The HCV NS3/4A protease – a chymotrypsin-like serine protease – is a prime therapeutic target that cleaves four known sites along the virally encoded polyprotein. The NS3/4A protease also hydrolyzes two human proteins, TRIF and MAVS, which are part of the innate immune system, thereby confounding the innate immune response to viral infection. In this study, we report that four chemically representative protease inhibitors – telaprevir, danoprevir, vaniprevir and MK-5172 – exhibit distinct susceptibilities to the protease variants R155K, A156T and D168A. To elucidate the underlying mechanism by which chemically diverse inhibitors bind to the wild-type protease and drug-resistant variants, crystal structures were determined for 16 inhibitor-protease complexes. These complexes include wild-type protease and resistant variants R155K, D168A and A156T each bound to telaprevir, danoprevir, vaniprevir and MK-5172, with resolutions ranging from 1.10–2.50 Å; S139A protease variants were used except for telaprevir, which requires covalent bond formation with the serine 139 for efficient binding.

Telaprevir lost potency against R155K compared to the wild-type protease, although the crystal structures of both complexes were very similar maintaining the covalent bond between the ketoamide moiety and the catalytic serine. R155K, however, lost interactions with D168, thereby disrupting the electrostatic network spanning R123, D168, R155 and D81, which is important for telaprevir binding. These rearrangements modulated the charge landscape along the protease surface, disrupting interactions with the adjacent P2 cyclopentylproline and P4 cyclohexylalanine moieties of telaprevir, consistent with previous modeling studies. Thus, while telaprevir's flexibility allows adaptation to D168A, it cannot accommodate the disruption by R155K or A156T. Telaprevir has reduced potency against R155K due to loss of van der Waals contacts but exhibits better potency against D168A as it allows tighter packing in the S2 subsite.

> GSHMASMKKKGSVVIVGRINLSGDTAYAQQTRGEEGCQETSQTGRDKNQVEGEVQIVSTATQTFLATSINGVLWTVYHGAGTRTIASPKGPVTQMYTNVDKDLVGWQAPQGSRSLTPCTCGSSDLYLVTRHADVIPVRRRGDSRGSLLSPRPISYLKGSSGGPLLCPAGHAVGIFKAAVSTRGVAKAVDFIPVESLETTMRSP>[2x]GPGFDYAVAMAKRNIVTATTSKGEFTMLGVHDNVAILPTHASPGESIVIDGKEVAILAAKALADQAGTNLEITIITLKRNEKFRDIRPHIPTQITETNDGVLIVNTSKYPNMYVPVGAVTEQGYLNLGGRQTARTLMYNFPTRAGQAGGVITCTGKVIGMHVGGNGSHGFAAALKRSYFTQSQGEIQWMRPSKEVGYPIINAPSKTKLEPSAFHYVFEGVKEPAVLTKNDPRLKTDFEEAIFSKYVGNKITEVDEYMKEAVDHYAGQLMSLDINTEQMCLEDAMYGTDGLEALDLSTSAGYPYVAMGKKKRDILNKQTRDTKEMQKLLDTYGINLPLVTYVKDELRSKTKVEQGKSRLIEASSLNDSVAMRMAFGNLYAAFHKNPGVITGSAVGCDPDLFWSKIPVLMEEKLFAFDYTGYDASLSPAWFEALKMVLEKIGFGDRVDYIDYLNHSHHLYKNKTYCVKGGMPSGCSGTSIFNSMINNLIIRTLLLKTYKGIDLDHLK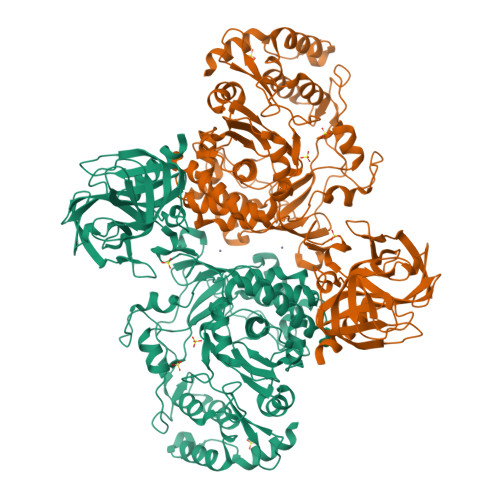MIAYGDDVIASYPHEVDASLLAQSGKDYGLTMTPADKSATFETVTWENVTFLKRFFRADEKYPFLIHPVMPMKEIHESIRWTKDPRNTQDHVRSLCLLAWHNGEEEYNKFLAKIRSVPIGRALDLPEYSTLYDRWLDSF>[3x]MEQDKILAHQASLNTKPSLLPPPVGNPPPVI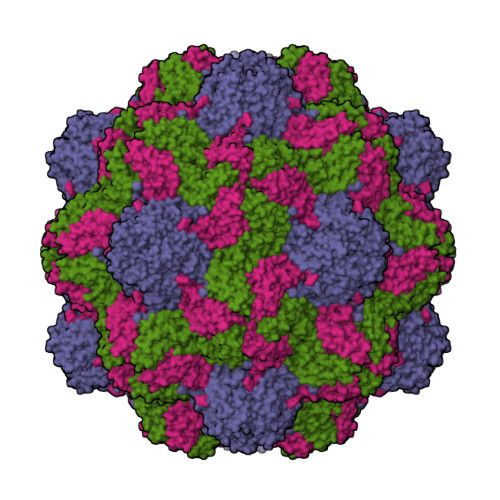SYPFQITLASLGTEDAADSVSIASNSVLATYTALYRHAQLKHLKATIHPTYMAPKYPTSVALVWVPANSTATSTQVLDTYGGLHFCIGGSVNSVKPIDVEANLTNLNPIIKASTTFTDTPKLLYYSKAQATAPTSPTCYLTIQGQIELSSPLLQASS> MTSVDCTAYGPELRALAARLPRTPRADLYAFLDAAHTAAASLPGALATALDTFNAEGSEDGHLLLRGLPVEADADLPTTPSSTPAPEDRSLLTMEAMLGLVGRRLGLHTGYRELRSGTVYHDVYPSPGAHHLSSETSETLLEFHTEMAYHRLQPNYVMLACSRADHERTAATLVA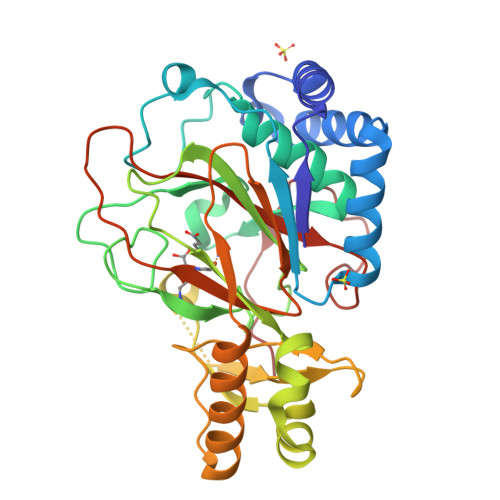SVRKALPLLDERTRARLLDRRMPCCVDVAFRGGVDDPGAIAQVKPLYGDADDPFLGYDRELLAPEDPADKEAVAALSKALDEVTEAVYLEPGDLLIVDNFRTTHARTPFSPRWDGKDRWLHRVYIRTDRNGQLSGGERAGDVVAFTPRG> SHGSHGMAVTKVTVDGIEFPPTITPPGSSKSLTLLGAGVRGIQIEGVEIKVTAIGIYAEPEVIASHLQKWKGKSASELVEDDGFFKDLVQAPVEKLARVTMLKPLTGAQYSGK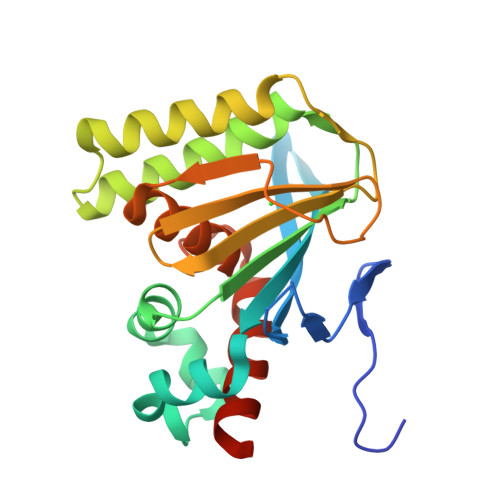VGENTKDALKALGKYSEAEEEALEEFREFFKTKSFPPGSTIFFHLSSPSTLQISFSTDGSLPEEAEATIENANFAAALLGTMLGKNGVSPSTKASVAEGISALLMKNKDEKEV>MSPAKDVKVYKKILEQNKDIQDLLDKIVFDAQHGQIWFDENRMLLMHTSILGFLRKDLYQMLGLERTKRFFIRCGYQAGMRDAEVTSKLRPNLNEAEAFMAGPQMHGIRGMVQVEVNELHLSHDLKQFYADFNWLNSFEAEVHLSEFGASDQPACWMLLGY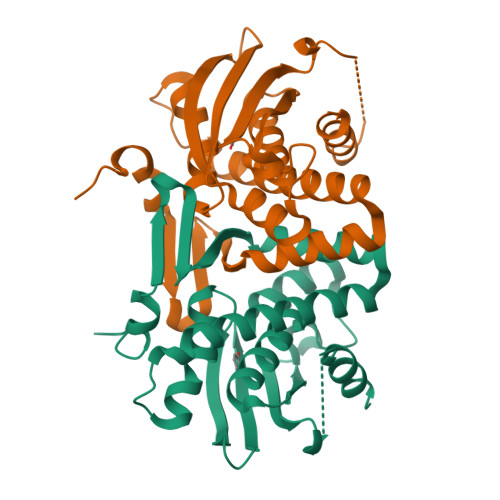ACGYSSFVMGQTIIYQETHCVAQGDEHCRIIGKPLSEWENADELIRFMSPDAVSDEIIALQAELNQLK[2x]> MEAPVYLCLLGNDPAPAYLGLKVVEREAGRVAKAVFYSFPAWNEEYGKKR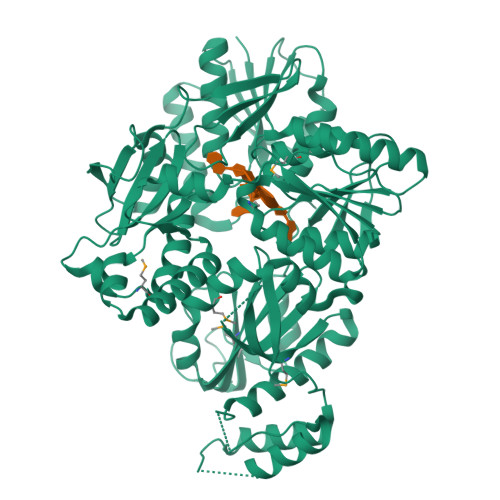QAFFRLLSEKGVLYEERPLEKGLEEAEAREVWVNLTGGAKYWAVRFLGHWRRPGARVFLVEGHRALEAPRALFLWPREEERSLEAEALTLEEYARLYLEPLGEAWERVSPPGAFPPGAQAARLPGREGGVFVVHRGLPYWYWVRPHLGGEAKDMSRKALSAFSGEAKRLGGQLCLPVVPYHKAHLRSRHPKERENVFARWRAWAREYGVFLVDPGRPLEEEVASLIKGKASKKALPLPQEGPLLLALVSEQAVPLYAAYLHAGPREVYLLTTPEMESRLRWAEAFFRGKGVRVHRSFLSGPWALREVRDLLAPVVEEALRRGHPVHANLNSGTTAMALGLYLALRDGARAHYLDGDRLLLLDGGEAEVPWEEGRPEDLLALRGYRFEEEYPDARPDPGLLALAEEILRRWDEVQTSWEASPLVRRFLKFWKKRFGQAFPPKRLSRLKGLPLEYAVYSHLNAHLAPKGGQARMGGHLVPLGGNEALAPQSTEVDGVFFHRGALWFVECKPTDEGLRERAPIMAELVRSVGGVEARGLMVARRWRGAPPPASPNLVYMALEGGEGVGVYRFPEELEKALSRNPAPRRGLE> DQNTEEMENLSDRVASDKAGNSATN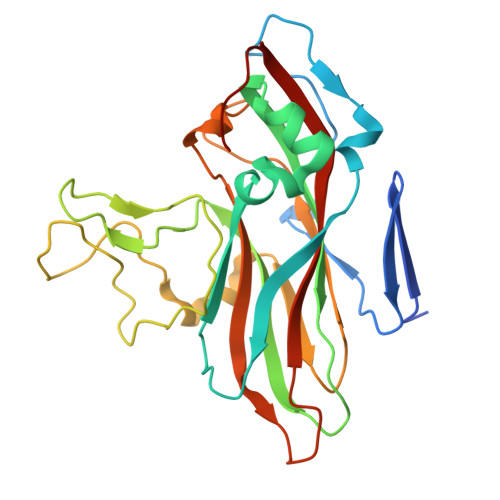TQSTVGRLCGYGEAHHGEHPASCADTATDKVLAAERYYTIDLASWTTTQEAFSHIRIPLPHVLAGEDGGVFGATLRRHYLCKTGWRVQVQCNASQFHAGSLLVFMAPEFYTGKGTKTGDMEPTDPFTMDTTWRAPQGAPTGYRYDSRTGFFAMNHQNQWQWTVYPHQILNLRTNTTVDLEVPYVNIAPTSSWTQHANWTLVVAVFSPLQYASGSSSDVQITASIQPVNPVFNGLRHETVIAQ> MSSVKISPLKDSEAFQSIKVGNNTLQTKIVYPPTTRFRALEDHTPSDLQLQYYGDRSTFPGTLLITEATFVSPQASGYEGAAPGIWTDKHAKAWKVITDKVHANGSFVSTQLIFLGRVADPAVMKTRGLNPVSASATYESDAAKEAAEAVGNPVRALTTQEVKDLVYEAYTN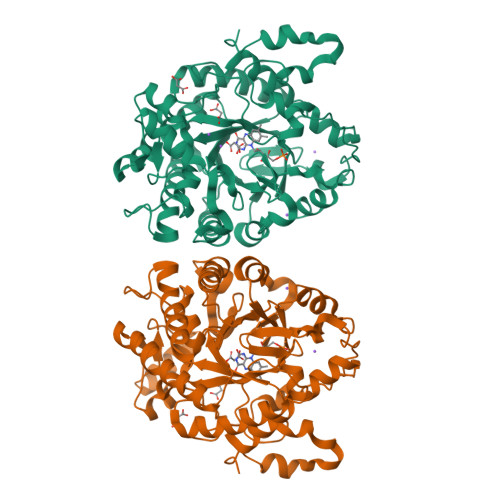AAQKAMDAGFDYIELHAAHGYLLDQFLQPCTNQRTDEYGGSIENRARLILELIDHLSTIVGADKIGIRISPWATFQNMKAHKDTVHPLTTFSYLVHELQQRADKGQGIAYISVVEPRVSGNVDVSEEDQAGDNEFVSKIWKGVILKAGNYSYDAPEFKTLKEDIADKRTLVGFSRYFTSNPNLVWKLRDGIDLVPYDRNTFYSDNNYGYNTFSMDSEEVDKELEIKRVPSAIEAL>[2x]MGHHHHHHHHHHHHSSG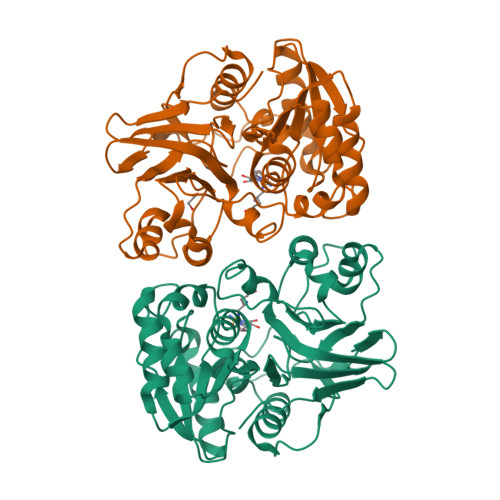HIDDDDKHMLEMIQSHPLLAAPLAVGDTIGFFSSSAPATVTAKNRFFRGVEFLQRKGFKLVSGKLTGKTDFYRSGTIKERAQEFNELVYNPDITCIMSTIGGDNSNSLLPFLDYDAIIANPKIIIGYSDTTALLAGIYAKTGLITFYGPALIPSFGEHPPLVDITYESFIKILTRKQSGIYTYTLPEKWSDESINWNENKILRPKKLYKNNCAFYGSGKVEGRVIGGNLNTLTGIWGSEWMPEIRNGDILFIEDSRKSIATVERLFSMLKLNRVFDKVSAIILGKHELFDCAGSKRRPYEVLTEVLDGKQIPVLDGFDCSHTHPMLTLPLGVKLAIDFDNKNISITEQYLSTEK> MEETRPIDGLTDEDIREILTRYKKIALVGASPKPERDANIVMKYLLEHGYDVYPVNPKYEEVLGRKCYPSVLDIPDKIEVVDLFVKPKLTMEYVEQAIKKGAKVVWFQYNTYNREASKKADEAGLIIVANRCMMREH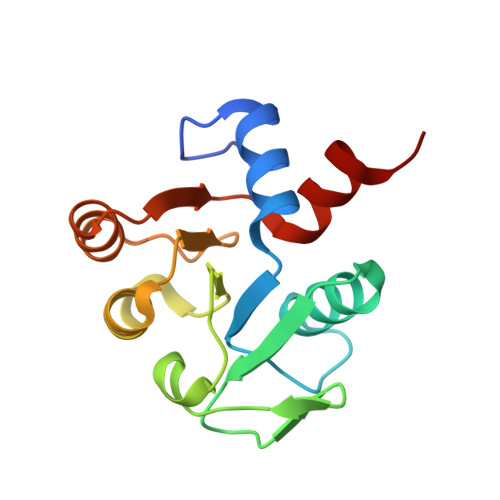ERLLGEK> QYSSNTQQGRTSIVHLFEWRWVDIALECERYLAPKGFGGVQVSPPNENVAIHNPFRPWWERYQPVSYKLCTRSGNEDEFRNMVTRCNNVGVRIYVDAVINHMCGNAVSAGTSSTCGSYFNPGSRDFPAVPYSGWDFNDGKCKTGSGDIENYNDATQVRDCRLSGLLDLALGKDYVRSKIAEYMNHLIDIGVAGFRIDASKHMWPGDIKAILDKLHNLNSNWFPEGSKPFIYQEVIDLGGEPIKSSDYFGNGRVTEFKYGAKLGTVIRKWNGEKMSYLKNWGE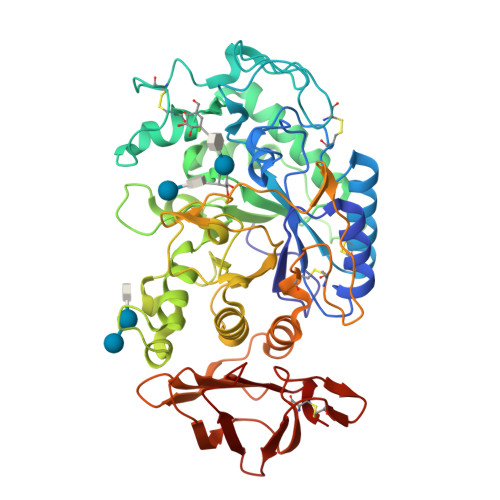GWGFMPSDRALVFVDNHDNQRGHGAGGASILTFWDARLYKMAVGFMLAHPYGFTRVMSSYRWPRYFENGKDVNDWVGPPNDNGVTKEVTINPDTTCGNDWVCEHRWRQIRNMVNFRNVVDGQPFTNWYDNGSNQVAFGRGNRGFIVFNNDDWTFSLTLQTGLPAGTYCDVISGDKINGNCTGIKIYVSDDGKAHFSISNSAEDPFIAIHAESKL> MSTFYQKPFLKLLDFTASELTALLQLAAKLKADKKN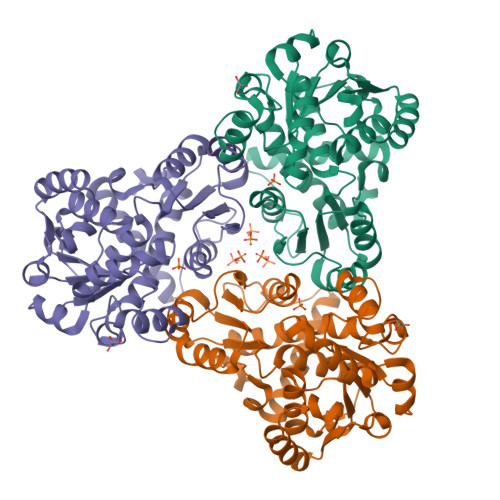GKEEQKLVGKNIALIFEKDSTRTRCSFEVAAYDQGARVTYLGSSGSQIGHKESIKDTARVLGRMFDGIQYRGYGQEIVETLAEYSGVPVWNGLTDEYHPTQLLADLLTMQEHLPGKAFNEMTLVYAGDARNNMGNSMLEAAALTGLDLRLVAPKACWPQAALVAECSAMAKKNGGAITLTEDIASGVKGADFIYTDVWVSMGEPKEKWAERIALLRDYQVNSQMMALTGNPQVKFLHCLPAFHDDETTLGKKMAEEYGLHGGMEVTDEVFESAASIVFDEAENRMHTIKAVMVATLSK2-methoxyphenyl beta-D-galactopyranoside | C13 H18 O7 | 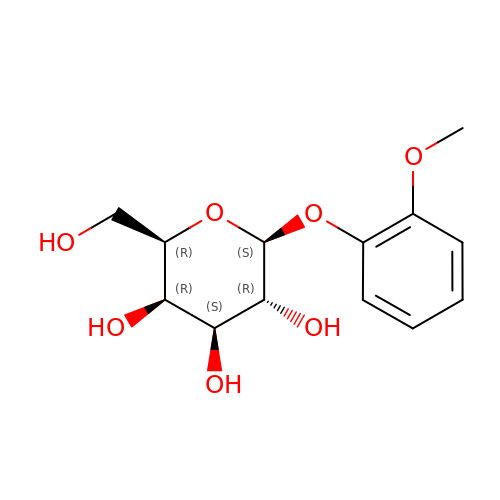WBZPEZUBVIAKKS-KSSYENDESA-N(2R,4S)-2-{(R)-carboxy[(phenylacetyl)amino]methyl}-5,5-dimethyl-1,3-thiazolidine-4-carboxylic 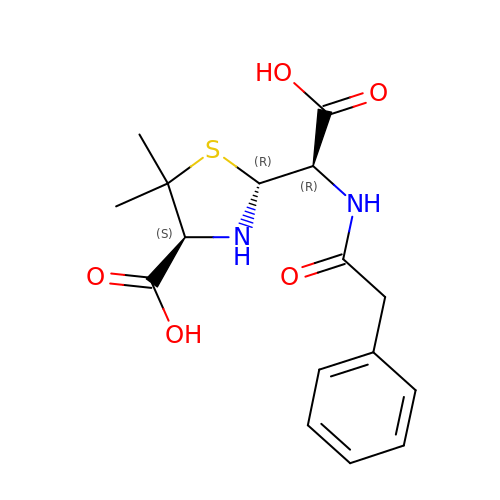acid | C16 H20 N2 O5 S | HCYWNSXLUZRKJX-RWMBFGLXSA-N> GPHMGEEAPPGVRSVKVVLVGDGGCGKTSLLMVFADGAFPESYTPTVFERYMVNLQVKGKPVHLHIWDTAGLDDYDRLRPLFYPDASVLLLCFDVTSPNSFDNIFNRWYPEVNHFCKKVPI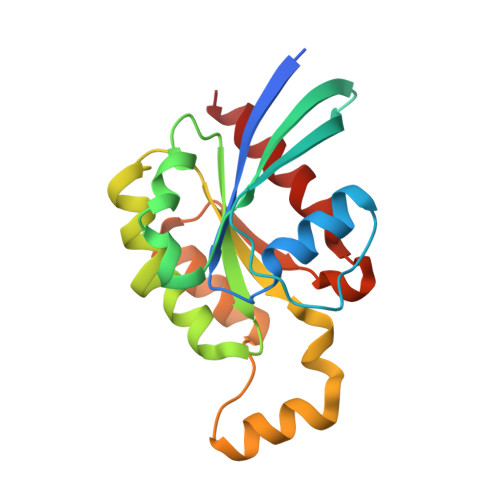IVVGCKTDLRKDKSLVNKLRRNGLEPVTYHRGQEMARSVGAVAYLECSARLHDNVHAVFQEAAEVALSSR>MTRQMILAVGQQGPIARAETREQVVVRLLDMLTKAASRGANFIVFPELALTTFFPRWHFTDEAELDSFYETE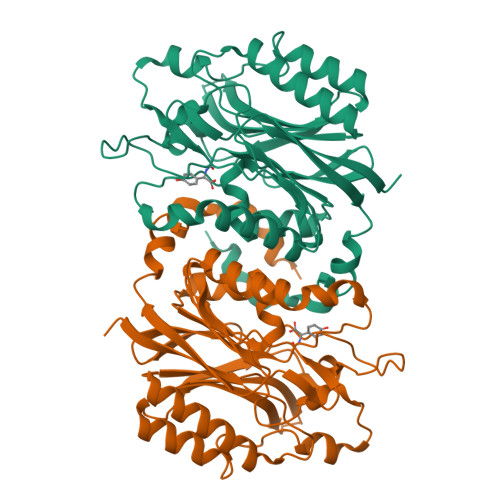MPGPVVRPLFEKAAELGIGFNLGYAELVVEGGVKRRFNTSILVDKSGKIVGKYRKIHLPGHKEYEAYRPFQHLEKRYFEPGDLGFPVYDVDAAKMGMFIANDRRWPEAWRVMGLRGAEIICGGYNTPTHNPPVPQHDHLTSFHHLLSMQAGSYQNGAWSAAAGKVGMEENCMLLGHSCIVAPTGEIVALTTTLEDEVITAAVDLDRCRELREHIFNFKQHRQPQHYGLIAEL[8x]>MVLRDDLDAVPGVPGV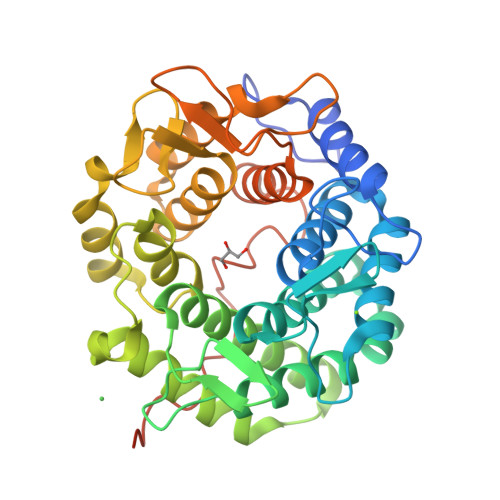LTPEQCRQTAQAIADAQEPSGALPWFEGGHTDPWDHVENAMALTVAGLLEPARAAFDWCRTTQRPDGSWPIQIRNGVVEDANSDSNFCAYVATGVWHHVLITGDRRFAETMWPVVAKAIDFVIDMQLPGGEIAWARSPSGLYEEALLTGCASIYHSIRCALALADYMGEPQPEWEVAVGRLGHAIAEHPEAFVTKDRWSMEWYYPVLGGALRGEAARARINRRWNDFVVPGLGIRCVDDRPWVTGAETCELVLALDAIGDLTRAHEQFAAMHHLREEDGSYWTGLVYDDGKRWPIERTTWTGAAMILAADALSRTTPGNGIFRGVDLPRGLEGEYDCACATSERKLAAALEHHHHHH[2x]> MKLSELFQMLSVGELSLIRTGNDGQGIRTQDYPKVIAQLNAGLTNLHARFPLLEKEVIIQQYEQISKYYLRS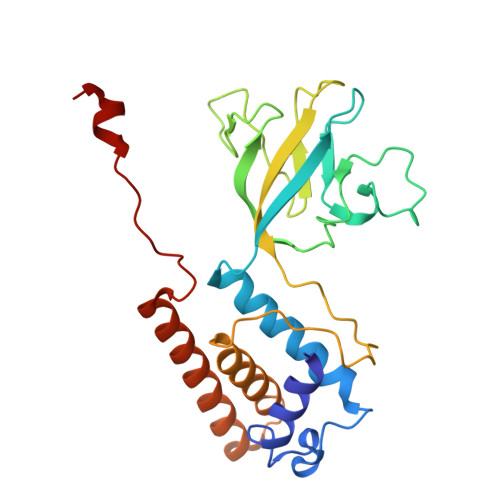EFAQMNTTSTEKYKYLMDSPTERFLDDVIRVERVFDECGCPLYLNNEPCCGSIVTPSFDCIQIVYPIETNALFVTYRANHPKIALTTTDLNTEVRIPASHEKALTYYIASQLYSNSPNPETAAKGVEWSQRFEAECTKIENLDLDNAHIAQTNVKPEMRGWV> ANKVIQLQKIFQSS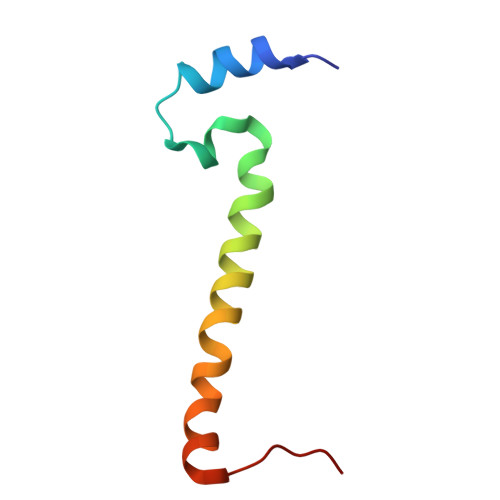TKPLWWRHPRSALYLYPFYAIFAVAVVTPLLYIPNAIRGIKAKKA> GSHSLRYFFTWSTAGSGIPEFVAVGYVDDQQFVQYDSDRKEMIPRQRWVKESEGPEYWERETQTLRGWEPWGKANIDILSKRTNQTGGIHTYQLMCGCELRDDGSSNTGFVQHAWDSTDFISLDKDKMVWVTPVTWGEITKNKWDRDMAFNQGTKGYLEGICIEWLQKYLKNGNVELRPVKPSVTFTSVRGNKQLSCVATGFYPHSIEVNLFRDSAKIDETESTGVRPNHDGSYQIHRSTE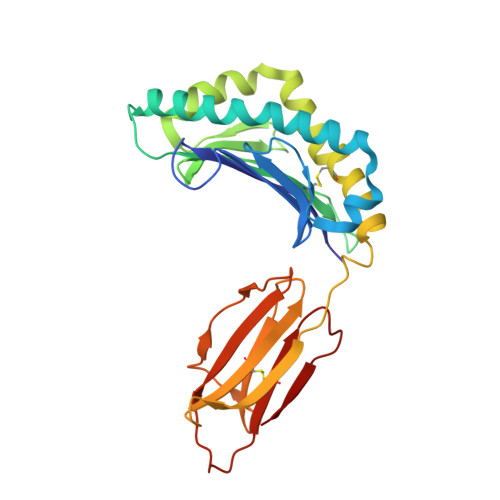FDPNSQAKYSCVVDHDGLGQQLVVFY> RQEFFWPEKARRTRVPLYQNSRPNLVYDQRFRRFMCMWYANGVQVFRPFSCRGRRGGRGKEGLPDGLGIGRGSG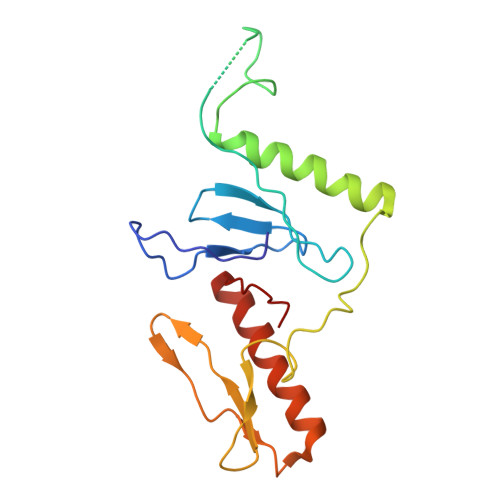TWERARAKAVVLLKQLQRQGHLDRLAKPDVTRSGVRGVYFDTEEKLWVATWNEHGLRRFKAFPTMEMGFDAAYQAAVAVRRQKLRENYIFSMQRNR>MAVKKIAIFGATGQTGLTTLAQAVQAGYEVTVLVRDSSRLPSEGPRPAHVVVGDVLQAADVDKTVAGQDAVIVLLGTRNDLSPTTVMSEGARNIVAAMKAHGVDKVVACTSAFLLWDPTKVPPRLQAVTDDHIRMHKVLRESGLKY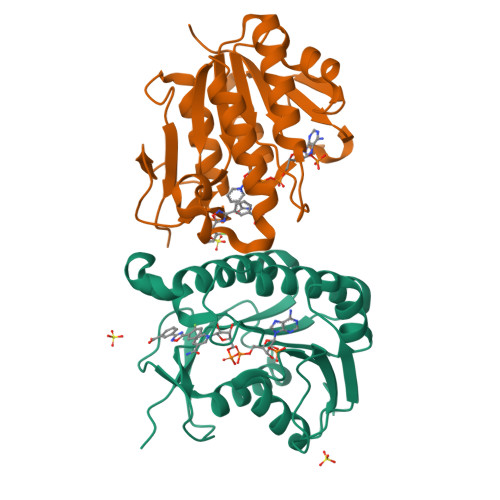VAVMPPHIGDQPLTGAYTVTLDGRGPSRVISKHDLGHFMLRCLTTDEYDGHSTYPSHQYQ[4x]> MRILAIDTATEACSVALWNNGTINAHFELCPREHTQRILPMVQEILAASGASLNEIDALAFGRGPGSFTGVRIGIGIAQGLALGANLPMIGVSTLATMAQGAWRKTGATRVLAAIDARM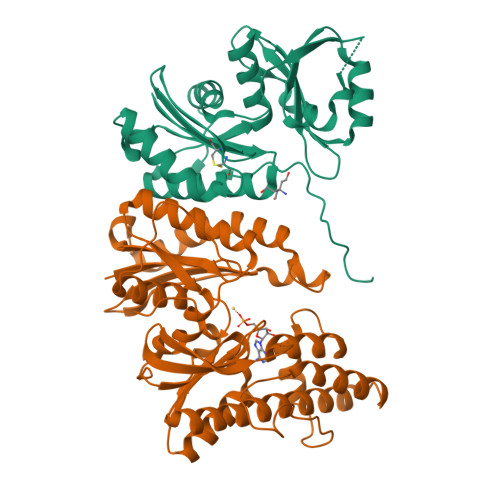GEVYWAEYQRDAQGVWQGEETEAVLKPERVGERLKQLSGEWATVGTGWSAWPDLAKECGLTLHDGEVSLPAAEDMLPIASQKLAAGETVAVEHAEPVYLRNEVAWKKLPG;> MRVLGIETSCDETGIAIYDDKKGLLANQLYSQVKLHADYGGVVPELASRDHVRKTVPLIQAALKEAGLTASDIDAVAYTAGPGLVGALLVGATVGRSLAFAWNVPAIPVHHMEGHLLAPMLEDNPPEFPFVALLVSGGHTQLISVTGIGQYELLGESIDDAAGEAFDKTAKLLGLDYPGGPMLSKMASQGTAGRFVFPRPMTDRPGLDFSFSGLKTFAANTIRSNGGDEQTRADIARAFEDAVVDTLMIKCKRALESTGFKRLVMAGGVSANRTLRAKLAEMMQKRRGEVFYARPEFCTDNGAMIAYAGMVRFKAGVTADLGVTVRPRWPLAELPAA> ANSLEPEPWFFKNLSRKDAERQ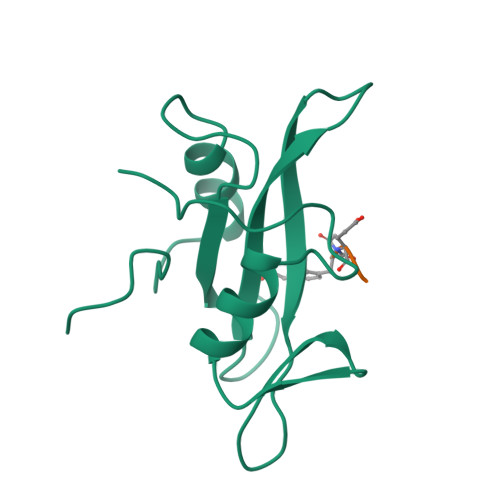LLAPGNTHGSFLIRESESTAGSFSLSVRDFDQNQGEVVKHYKIRNLDNGGFYISPRITFPGLHELVRHYTNASDGLCTRLSRPCQT;> XFEEI> MVARPKSEDKKQALLEAATQAIAQSGIAASTAVIARNAGVAEGTLFRYFATKDELIN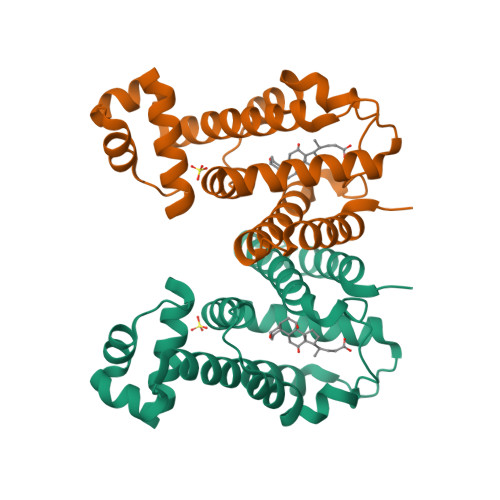TLYLHLKQDLCQSMIMELDRSITDAKMMTRFIWNSYISWGLNHPARHRAIRQLAVSEKLTKETEQRADDMFPELRDLCHRSVLMVFMSDEYRAFGDGLFLALAETTMDFAARDPARAGEYIALGFEAMWRALTREEQ>[4x]MTQERKVALVTGASRGIGAAIAQQLIQDGYFVVGTATSESGAQKLTDSFGEQGAGLALDVRNLDEIEAVVSHIEQNYGPVLVLVNNAGITKDNLLLRMSEDDW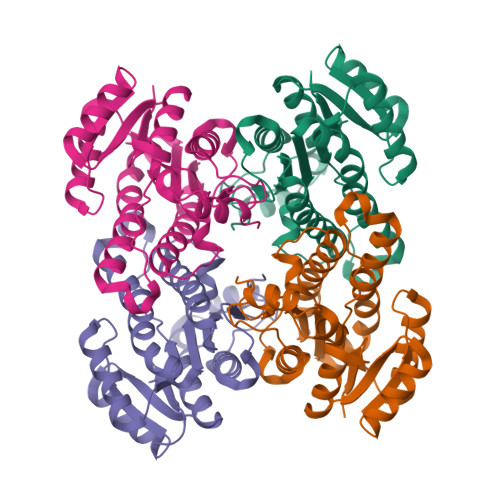DDILNIHLKAVYRLSKRVLKGMTKARFGRIINISSVVAHFANPGQANYSAAKAGIEAFSRSLAKEMGSRQITVNSVAPGFIATEMTDALSEDIRKKMSDQVALNRLGEPQDIANAVSFLASDKAGYITGTVLHVNGGLYMA>GSSAVNQENERLMEEYERLASELLEWIRRTIPWLENRTPEKTMQAMQKKLEDFRDYRRKHKPPKVQEKCQLEINFNTLQTKLRISNRPAFMPSEGKMVSDIAGAWQRLEQAEKGYEEWLLNEIRRLERLEHLAEKFRQKASTHETWAYGKEQILLQKDYESASLTEVRALLRKHEAFESDLAAHQDRVEQIAAIAQELNELDYHDAVNVNDRCQKICDQWDRLGTLTQKRREALERMEKLLETIDQLHLEFAKRAAPFNNWMEGAMEDLQDMFIVHSIEEIQSLITAHEQFKATLPEADGERQSIMAIQNE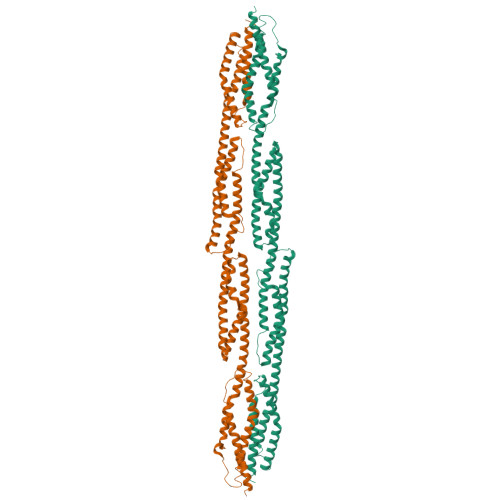VEKVIQSYNIRISSSNPYSTVTMDELRTKWDKVKQLVPIRDQSLQEELARQHANERLRRQFAAQANAIGPWIQNKMEEIARSSIQITGALEDQMNQLKQYEHNIINYKNNIDKLEGDHQLIQEALVFDNKHTNYTMEHIRVGWELLLTTIARTINEVETQILTRD[2x]5-methylidene-3-(methylsulfanyl)-2-benzothiophen-4(5H)-one 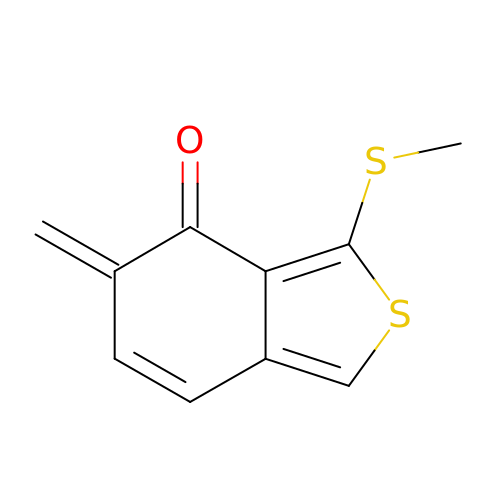| C10 H8 O S2 | BRJSKZMFXIHQOD-UHFFFAOYSA-N> FHLTTRNGEPHMIVSRQEKGKSLLFKTEDGVNMCTLMAMDLGELCEDTITYKCPFLKQNEPEDIDCWCNSTSTWVTYGTCTTTGEHRREKRSVALVPHVGMGLETRTETWMSSEGAWKHAQRIETW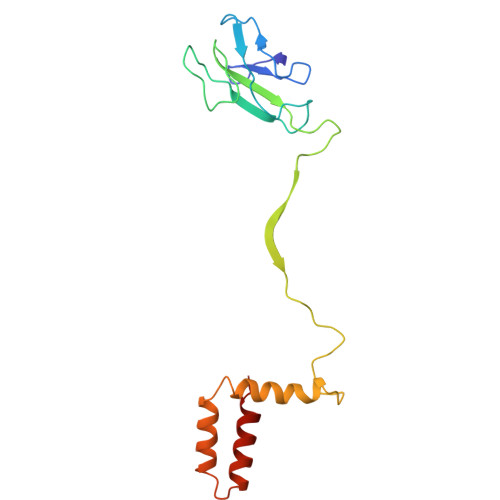ILRHPGFTIMAAILAYTIGTTHFQRALIFILLTAVAPSMT> MLKVNEFETDTDLRGNINYLFNDEANVVYTYDGTESDLLQNVNEVSKYIEHHMDYQRPRLKVLSDYYEGKTKNLVELTRRKEEYMADNRVAHDYASYISDFINGYFLGNPIQYQDDDKDVLEAIEAFNDLNDVESHNRSLGLDLSIYGKAYELMIRNQDDETRLYKSDAMSTFIIYDNTVERNSIAGVRYLRTKPIDKTDEDEVFTVDLFTSHGVYRYLTNRTNGLKLTPRENSFESHSFERMPITEFSNNERRKGDYEKVITLIDLYDNAESDTANYMSDLNDAMLLIKGNLNLDPVEVRKQKEANVLFLEPTVYVDAEGRETEGSVDGGYIYKQYDVQGTEAYKDRLNSDIHMFTNTPNMKDDNFSGTQSGEAMKYKLFGLEQRTKTKEGLFTKGLRRRAKLLETILKNTRSIDANKDFNTVRYVYNRNLPKSLIEELKAYIDSGGKISQTTLMSLFSFFQDPELEVKKIEEDEKESIKKAQKGIYKDPRDINDDEQDDDTKDTV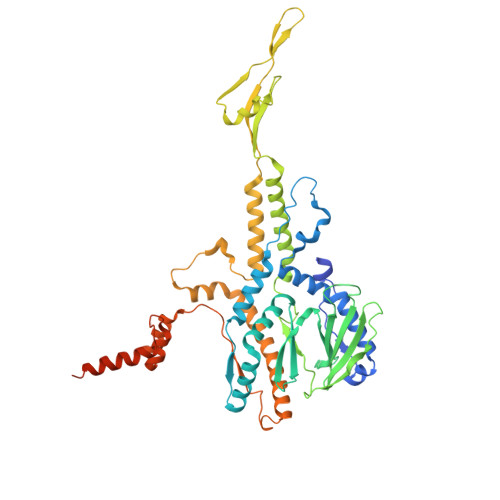DKKE>GIDPFTMSLQEPVSPVEESPTSTADRIADLAARHEEAVVLAEKKAADRQHLKGKLTARARIDLLLDPGSFVELDEFVRHRTVEAGIPRPYGDGVVTGHGTIDGRQVCVFSHDFTTLGGSMGEAFGSKVVKIYDFAMSVGCPVIGINDSGGARIQEGVMSIAYYTELGVRNVHSSGVIPQISLIMGPCAGGSVYSPALTDFTVMVKDISYMFVTGPEVVSAVMGEQVTAEQLGGPAVHAEVSGNAHYVGDDEQDAISWVQTLLGYLPPNNLDPAPVYDHDCAPGITEADLALDTVIPDSEQQVYDMADVITAVLDDGDYLEIHPDFARNIICALGRVEGHSVAVVANQPRHLAGVLDIDASEKAARFIRFCDSFNIPVLTFMDVPGYLPGVGQEHQGIIRRGIKLFYAYAESTVPKITVITRKAYGGGYAVMGSRQIGADRVMAWPTAEIAVMGANSAVPILHRRELAAVPPEERAAVKENLVDDYRRRFGNPYEAAAHGYVDMVISPSRTRYEVARA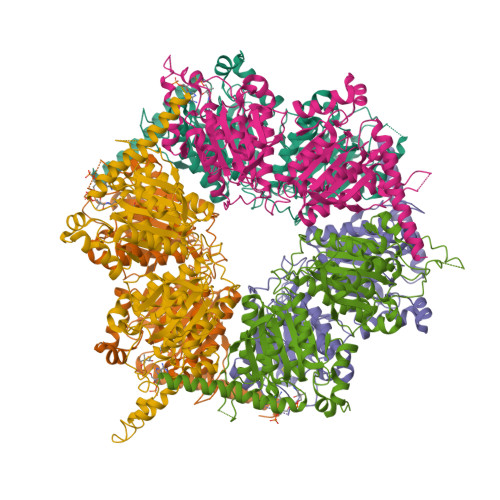LASLRNKRQARPARKHGNIPL[6x]>MGSSHHHHHHSQDPNSSSMGQDGQQIRRDKLIIDTDPGIDDSMTILMAFRAPSVEIIGLTTIFGNVDTKGATRNALLLCERAGCPEVPVAEGSHEPLKGGKPRVADFVHGSDGIGNLFLPAPSAKKVEESAADFLINKVSEFPGEVSVLALGPLTNVALAIKRDPSFASKVKKIVVLGGAFFAAGNVNPAAEANIHGDPEAADIVFT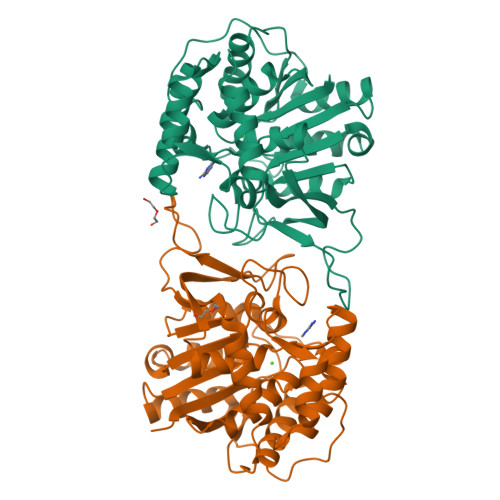SGADIVVVGINITTQVCLTDEDLLELRNSKGKHAAFLYEMCKFYRDWHAKSDGFHGIFLHDPVSFTAVLHPEYFTFKKGVVRVETQGICTGHTLMDQGLKKWNSENPWSGYKPISVAWTVDVPKVISFIKKLLMAP[4x]>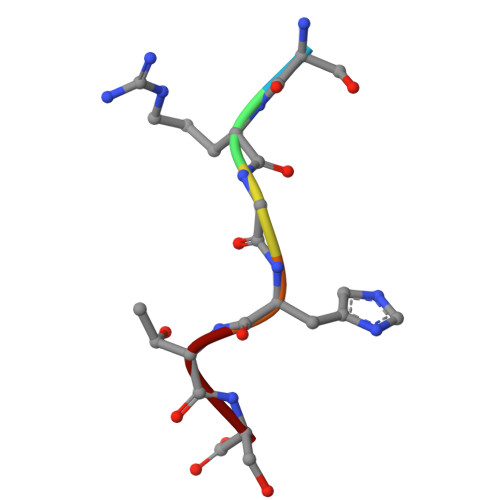 SRGHTS cis-4-[3-amino-6-(3-cyclopropylthiophen-2-yl)pyrazin-2-yl]cyclohexanecarboxylic acid | C18 H21 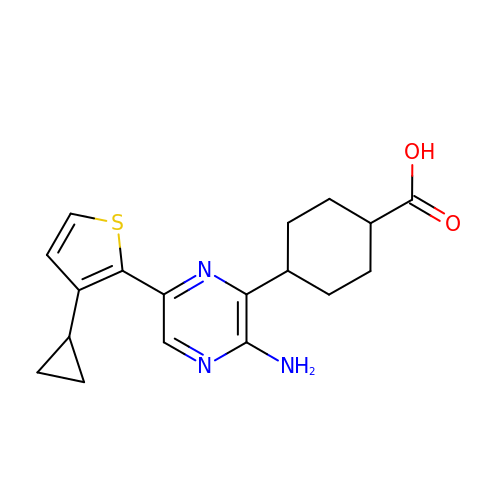N3 O2 S | UESQMXBXMMVHBA-TXEJJXNPSA-N> GVMTDVHRRFLQLLMTHGVLEEWDVKRLQTHCYKVHDRNATVDKLEDFINNINSVLESLYIEIKRGVTEDDGRPIYALVNLATTSISKMATDFAENELDLFRKALELIIDSETGFASSTNILNLVDQLKGKKMRKKEAEQVLQKFVQNKWLIEKEGEFTLHGRAILEMEQYIRETYPDAVKICNICHSLLIQGQSCETCGIRMHLPCVAKYFQSNAEPRCPHCNDYWPHEIPKVFDPE;> GPRSQKQLELKVSELVQFLLIKDQKKIPIKRADILKHVIGDYKDIFPDLFKRAAERLQYVFGYKLVELEPKSNTYILINTLEPVEEDAEMRGDQGTPTTGLLMIVLGLIFMKGNTLKETEAWDFLRRLGVYPTKKHLIFGDPK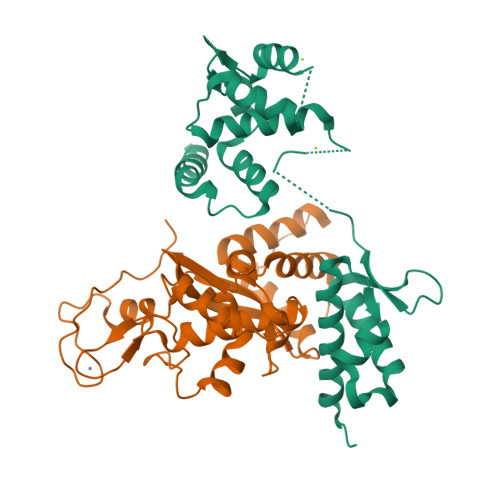KLITEDFVRQRYLEYRRIPHTDPVDYEFQWGPRTNLELSKMKVLKFVAKVHNQDPKDWPAQYCEALADEENRAR Here, we report two crystal structures of this novel protein family, a circularly permuted imelysin (with the GxHxxE motif) from Bacteroides ovatus (PIBO) and an imelysin-like protein (with a variant GxxxxE motif) from Psychrobacter arcticus 273-4 (IPPA). The PIBO monomer is a V-shaped, all helical structure consisting of two domains, D1 (residues 33–90 and 244–384) and D2 (residues 91–243), with molecular dimensions of 73 Å×55 Å×42 Å. The functional site of PIBO is likely located at the domain interface and supported by the clustering of conserved residues, including the buried GxHxxE motif. As a result, our structural evidence clearly argues against PIBO being a metallopeptidase.

The asymmetric unit (asu) of the final model contains two monomers (A, residues 33–384, and B, residues 31–384), 1191 water molecules and other solvent molecules that were present in the purification, crystallization or cryo-protection reagents, including three magnesium ions, two chloride ions, and seven ethylene glycol molecules. The two monomers in the asu of crystal form 1 of PIBO are essentially identical with an rmsd of 0.5 Å for 352 Cα atoms. These two monomers are also very similar to the monomer in crystal form 2, except for a region between residues 329 and 365 (rmsd 4.0 Å overall, 0.63 Å if residues 329–365 are omitted). In crystal form 1, a magnesium ion, which is present in the crystallization solution, is found at the mouth of the pocket. However, it is coordinated by water molecules only, and does not directly interact with any side-chain atoms. Mg2+ was present in the crystallization buffer; however, neither residue is involved in the binding of the Mg2+ identified in the crystal structure. This lack of observed metal binding in this region, despite its presence in solution, casts doubt on PIBO's ability to bind divalent ions directly. The αO-αR insert (defined as the region between αO and αR) of PIBO adopts different conformations in the two crystal forms. The αO-αR insert in crystal form 1 contains two helices (αP and αQ), as well as a short 310 helix. Helix αQ (residues 355–362) interacts with helix αO, while the 310 helix and the loops connecting to it lie in the interface between helix A and helices αO and αR.

>[2x]GSDDDNPTVDPANIDYTPENASSWHNYMRNVAALLKTDATNLYNAWNSSYKGGESYASLFKAHSGSPYASALSCVEEIVDKCAEIANEVGTAKIGDPYNLYKAGNTEEALYAVESWYSWHSRDDYTNNIYSIRNAYYGSLDGNINANSLSTVIAGANSSLDTKIKNAIQKAAKAIQDIPQPFRNHIPSNETVAAMDACAELESILKNDLKSYIANNSNNINTDAVLNPVVTQYVDAVVVPTYKSLKEKNDALYNAVIVLADNPSNSAFETACDAWITAREPWEKSEAFLFGPVDEMGLDPNMDSWPLDQNAIVQILNSQSWSDLEWSEGDDEAAVESAQNVRGFHTLEFLLYKNGEPRKVQ>[14x]MAIAQLATEYVFSDFLLKEPTEPKFKGLRLELAVDKMVTCIAVGLPLLLISLAFAQEISIGTQISCFSPSSFSWRQAAFVDSYCWAAVQQKNSLQSESGNLPLWLHKFFPYILLLFAILLYLPPLFWRFAAAPHICSDLKFIMEELDKVYNRAIKAAKSARDLDMRDGACSVPGVTENLGQSLWEVSESHFKYPIVEQYLKTKK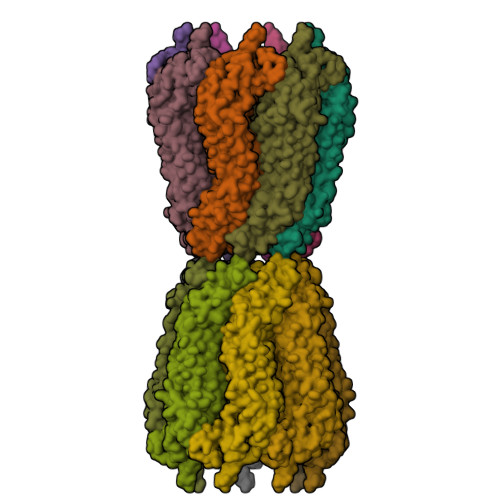NSNNLIIKYISCRLLTLIIILLACIYLGYYFSLSSLSDEFVCSIKSGILRADSTVPDQFQCKLIAVGIFQLLSVINLVVYVLLAPVVVYTLFVPFRQKTDVLKVYEILPTFDVLHFKSEGYNDLSLYNLFLEENISEVKSYKCLKVLENIKSSGQGIDPMLLLTNLGMI>GSHMRPFLPKKKQQKDSLINLKIQKENPKVVNEINIEDLSLTKAAYCRCWRSKTFPACDGSHNKHNELTGDNVGPLI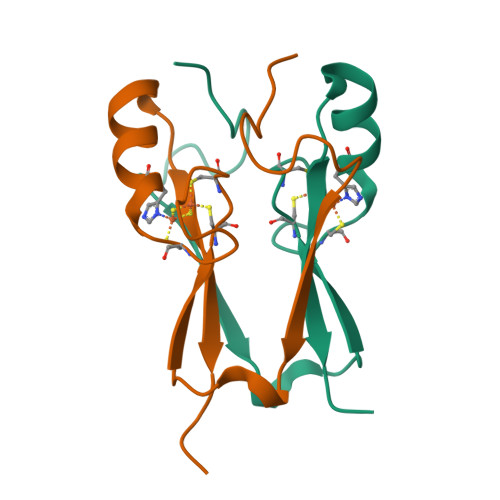LKKKEV[2x]>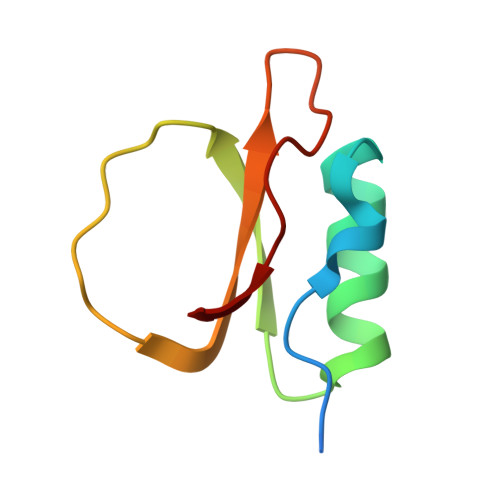 GHMASQCPVKNSWPELVGTNGDIAAGIIQTENANVKAIVVKEGLPITQDLNFNRVRVFVDENRVVTQVPAIG>GGLTLKVVTVLEEPFVMVAENILGQPKRYKGFSIDVLDALAKALGFKYEIYQAPDGRYGHQLHNTSWNGMIGELIS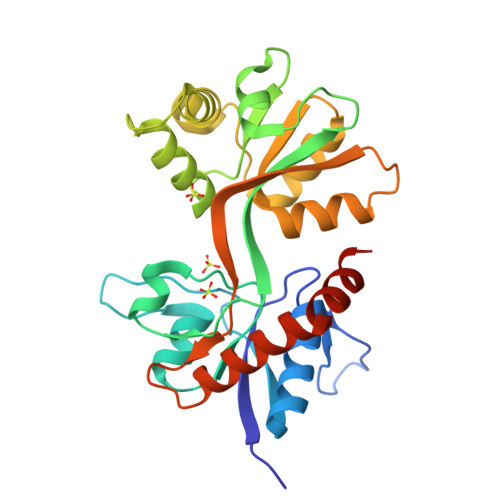KRADLAISAITITPERESVVDFSKRYMDYSVGILIKKGTPVRTFQDLSKQLEMSYGTVRDSAVYEYFRAKGTNPLEQDSTFAELWRTISKNGGADNCVSNPSEGIRKAKKGNYAFLWDVAVVEYAALTDDDCSVTVIGNSISSKGYGIALQHGSPYRDLFSQRILELQDTGDLDVLKQKWWPHTGRCDLT[2x]4-(2-aminoethyl)phenol | C8 H11 N O | 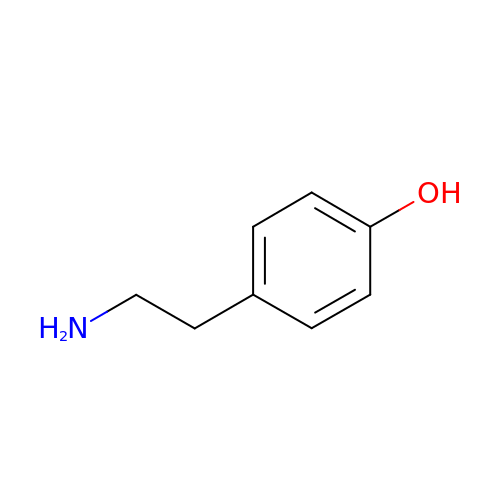DZGWFCGJZKJUFP-UHFFFAOYSA-N>[2x]APITAYSQQTRGLLGCIITSLT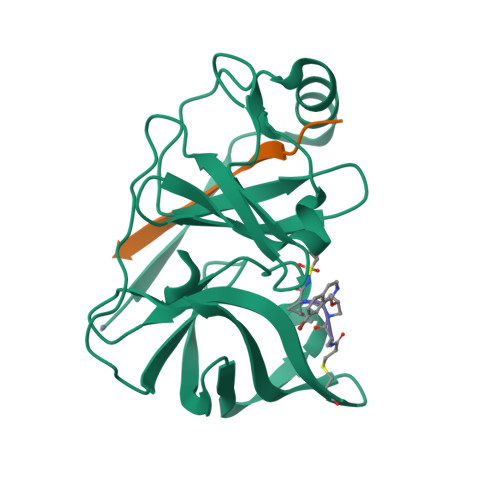GRDKNQVDGEVQVLSTATQSFLATCVNGVCWTVYHGAGSKTLAGPKGPITQMYTNVDQDLVGWPAPPGARSMTPCTCGSSDLYLVTRHADVIPVRRRGDSRGSLLSPRPVSYLKGSSGGPLLCPSGHVVGIFRAAVCTRGVAKAVDFIPVESMETTMRSPVFTDN;>KGSVVIVGRIILSGRK[2x]> GPLGSAPVRSLNCTLRDSQQK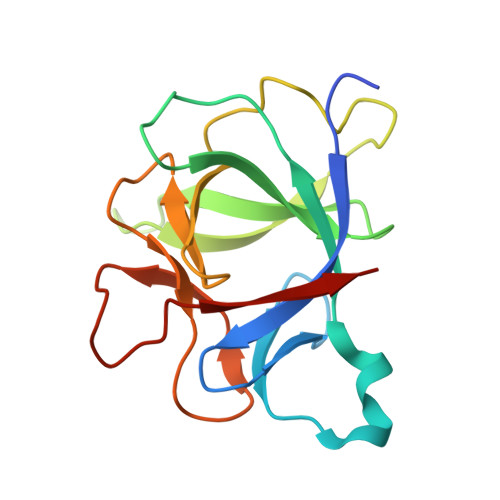SLVMSGPYELKALHLQGQDMEQQVVFSMSFVQGEESNDKIPVALGLKEKNLYLSCVLKDDKPTLQLESVDPKNYPKKKMEKRFVFNKIEINNKLEFESAQFPNWYISTSQAENMPVFLGGTKGGQDITDFTMQFVSS> MAATAAEAVASGSGEPREEAGALGPAWDESQLRSYSFPTRPIPRLSQSDPRAEELIENEEPVVLTDTNLVYPALKWDLEYLQENIGNGDFSVYSASTHKFLYYDEKKMANFQNFKPRSNREEMKFHEFVEKLQDIQQRGGEERLYLQQTLNDTVGRKIVMDFLGFNWNWINKQQGKRGWGQLTSNLLLIGMEGNVTPAHYAEQQNFFAQIKGYKRCILFPPDQFECLYPYPVHHPCDRQSQVDFDNPDYERFPNFQNVVGYETVVGPGDVLYIPMYWWHHIESLLNGGITITVNFWYKGAPTPKRIEYPLKAHQKVAIMRNIEKMLGEALGNP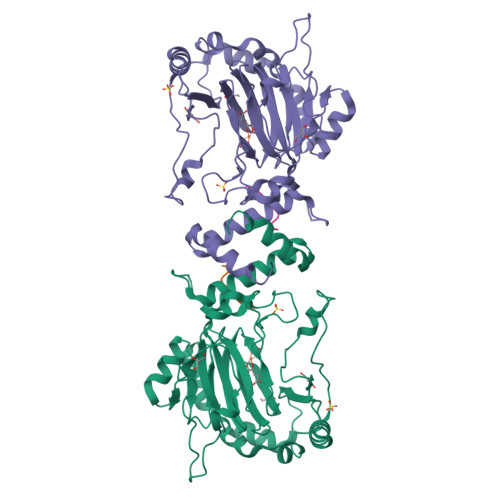QEVGPLLNTMIKGRYN;> SMDESGLPQLTSYDCEVNAPIQGSRNLLQGEELLRALDQVN> SNATDSTVSTDPVTLNTEKTTLDQDVVINGDNKITAVTIETSDSDKDLNVTFGGHDITATSTVNQDFVEGVKVSGNKNVVINATDSTITAQGEGTYVRTAMVIDSTGDVVVNGGNFVAKNEKGSATGISLEATTGNNLTLNGTTINAQGNKSYSNGSTAIFAQKGNLLQGFDGDATDNITLADSNIINGGIETIVTAGNKTGIHTVNLNIKDGSVIGAANNKQTIYASASAQGAGSATQNLNLSVADSTIYSDVLALSESENSASTTTNVNMNVARSYWEGNAYTFNSGDKAGSDLDINLSDSSVWKGKVSGAGDASVSLQNGSVWNVTGSSTVDALAVKDSTVNITKATVNTGTFASQNGTLIVDASSENTLDISGKASGDLRVYSAGSLDLINEQTAFISTGKDSTLKATGTTEGGLYQYDLTQGADGNFYFVKNTHKASNASSVIQAMAAAPANVANLQADTL

Autotransporters (ATs) are the largest group of outer membrane and secreted proteins in bacteria and play important roles in virulence, including promoting adhesion. UpaB is an AT that mediates UPEC adherence to extracellular matrix (ECM) proteins and enhances UPEC colonisation of the urinary tract. UpaB is composed of an N-terminal signal sequence (residues 1–37), an α-domain (residues 38–500) and a β-domain (residues 501–776). Here we determine the structure of UpaB at high resolution and reveal that it adopts a unique architecture potentially comprising two distinct binding sites.

The αUpaB crystal structure was solved to 1.9 Å resolution (crystallographic Rfactor of 17.5%; Rfree 21.8%). The structure was solved from a xenon derivative by single isomorphous replacement with anomalous scattering. The crystal structure of αUpaB exhibited a right-handed three-stranded β-helix consisting of 13 turns, with each triangular turn containing three faces, F1, F2 and F3 faces. The interior of the β-helix is packed mostly by long stacks of aliphatic residues, whereas the exterior is largely acidic in nature. At the C-terminus of the β-helix, αUpaB forms a two-stranded β-sandwich that is capped by a three-stranded β-meander motif. However, the most striking feature of the αUpaB β-helix is the extended β-strands within turns 6–10, which reach up to 32 Å in length. The β-strand extensions contributed by turns 6–10 and the long loops protruding between turns 2–6 form a long hydrophilic groove 11 Å wide and 12.5 Å deep on the F1 face of αUpaB. Indeed, we identified electron density associated with the αUpaB lysine pair likely to be a bound calcium. Similar to other lyases, this calcium ion would be held in place by the neighbouring αUpaB Glu 314 and Asn 316 residues. Substitution of residues D116, D119, N146, N175, D217, K245, D246, D281, R310 and D336 on the F2 face to alanine (αUpaB_S1) caused almost complete loss of FN binding as determined by ELISA, while maintaining the correct secondary structure of αUpaB_S1 based on circular dichroism spectroscopic analysis and displaying a behaviour in solution similar that of the native protein. This result mapped the FN-binding site to a ladder of charged/polar residues that are contributed from β-strands or loops in consecutive rungs of the αUpaB β-helix.Enzymes of the vanillyl alcohol oxidase/p-cresol methyl hydroxylase (VAO/PCMH) superfamily are found across all kingdoms where they perform a range of metabolic functions. These flavoproteins share a conserved FAD-binding domain and a more variable substrate-binding domain that enables interactions with a range of substrates. One of these, the 4-phenol oxidases/dehydrogenases, catalyzes the oxidation of para-substituted phenolic compounds. A fundamental distinction is that the oxidases efficiently react with oxygen producing hydrogen peroxide whereas the dehydrogenases hardly react with oxygen and typically employ other proteins, such as cytochrome c, as acceptors.

We further studied the P151G mutation to assess the effect of removing en bloc the side chain, and P151N and P151T to test the introduction of hydrogen-bonding groups. The P151G mutation was found to elicit the same oxidase-activating effect of P151L whereas P151T and P151N conserve the properties of a dehydrogenase. Spectrophotometric measurements confirmed that the vanillyl alcohol-reduced P151N and P151T proteins are hardly re-oxidized by molecular oxygen though they retain dehydrogenase activity while P151G can effectively turn over using oxygen as co-substrate and the product is formed. Conversely, in the dehydrogenase variants (P151N and P151T), like in the wild-type structure, the loop obstructs the access to the N5 atom. In particular, Thr151 of P151T adopts a cis conformation as observed for the wild-type Pro151. Conversely, no tunnels are present in the wild type and the dehydrogenase mutants where the flavin re face remains fully shielded by residue 151 and Trp153.

>[3x]MAAPLPEGVSAEAMSSALDRFARIVGADWVFTEDKITPYEDPYTISNDETEHRPYAAVAPASTEEVQEIVRVANEFGVPLWPVSRGKNFAYGGAAPVMSGTVVLDMNRMNRILEVNEEFGYALVEPGVSYFELYDYIQEKGLKLWIDVPDTGWGSVVGNALDHGIGYTPYGDHFAMQCGMEVVLPNGEVVRTGMGAMPGNNTWQLFKYGYGPYVDGIFSQSNFGVVTKMGIWLMPEPAGYRPYLITFENEDDIETVTERLRPLKVAGVIQNGATVRSLVLDAAITRTKSQYYDGDGPIPPSVAKTMMADLDLGMWNFCGALYGPPPVMDTLWTAIRDSFADIPGVKFYFPEDRRHKVDLLLHRAETMKGVPKLTEFNFLNWDGGGGHVGFSPVSPITGKDAIKQYNMVSSRVREYGFDYMGLLAIGWRDLHHVTVIVYDKTDPDERKKLDELFNILVDEAAAEGYGEYRTHIRYMDRIAKTYSWNDNALWKMHETIKDALDPNGILAPGKSGIWGKNRRKA>GEKGDWAQFGRYAEANKTVKVPSNVVFMGNSITDGWWPADSTFFIRNNFVDRGISGQTTSEMLVRFRQDVINLKPKAVVILAGINDIAHNNGVIALENVFGNLVSMAELAKANHIKVIFCSVLPAYDFPWRPGMQPADKVIQLNKWIKEYADKNGLTYVDYHS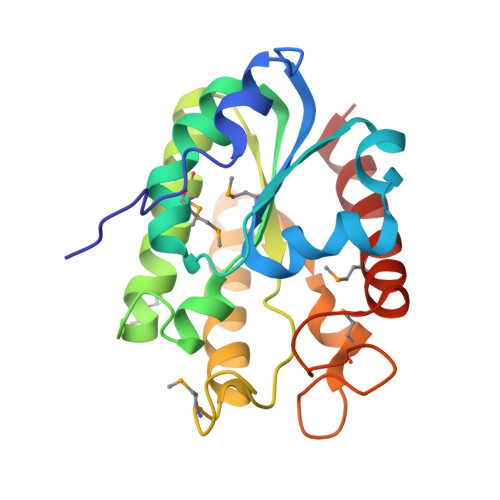AMKDERNGLPANLSKDGVHPTLEGYKIMEKIVLEAIHKTVK[4x]Sdk1 and Sdk2 are single-pass transmembrane proteins, with extracellular regions composed of 6 N-terminal immunoglobulin (Ig) domains followed by 13 fibronectin type III (FNIII) domains, and a relatively short intracellular domain terminating in a Postsynaptic density/Discs Large/ZO-1 (PDZ) binding motif. Here, we report the crystal structures of cell-cell adhesive homophilic dimers of mouse Sdk1 and Sdk2, each mediated by the four N-terminal Ig domains. These four domains adopt a horseshoe conformation, like many other IgSF cell-cell recognition proteins, but they interact in a unique back-to-back anti-parallel manner not previously observed. Overall, our data suggest a model in which Sdks form cis dimers on isolated cell surfaces, which dissociate to form trans dimers through the same interface when contact is made to a cell surface expressing the cognate Sdk.

The Sdk1Ig1–5 structure showed that Ig5 extends laterally from the horseshoe with a 54° deviation from linearity with Ig4. This angle is maintained in both independent Ig1–5 chains observed in the crystal structure. The linker between Ig4 and Ig5 is only one amino acid (N379) and there is a small Ig4:Ig5 interface with a buried surface area (BSA) over both domains of ~370 Å2. This interface—involving the linker region, the Ig4 AB loop and the Ig5 BC loop—likely provides rigidity to the Ig4–Ig5 junction. Consistent with the AUC results of the wild-type Sdk1 and Sdk2, the crystal structures show a dimeric arrangement of molecules, consisting of symmetrical back-to-back interactions (convex-face to convex-face) between the Ig1–4 horseshoe regions of the individual protomers, with Ig5 making no contacts in the Sdk1Ig1–5 dimer. (A) Surface view of the Sdk1Ig1–5 structure showing the back-to-back horseshoe-mediated dimer observed in the crystal structure. The positioning of Ig6 is therefore unknown, however, since Ig5 projects away from the dimer interface it is unlikely Ig6 would be able to contribute to the dimer observed in the crystal structures, which is described in detail below. (G) Our data suggest Sdk dimerizes using the crystallographically-determined interface, both between molecules emanating from opposing cell surfaces (in trans)—mediating cell-cell interactions—and between molecules emanating from the same cell surface (in cis)—mediating Sdk clustering. These interactions are shown schematically, using the Sdk1Ig1–5 crystal structure to illustrate the dimer interaction.

>[2x]GPALAQDDVAPYFKTEPGLPQIHLEGNRLVLTCLAEGSWPLEFKWIRNDSELTTYSSEYKYIIPSLQKLDAGFYRCVVRNRMGALLQRKSEIQVAYMGNFMDTDQRKTVSQGHAALLNLLPIVSCPQPQVTWFREGHKIIPSSRIAITLENQLVILATTASDAGAYYVQAVNEKNGENKTSPFIHLSVARDTGTHEAMAPIIVVAPGNRSVVAGSSETTLECIANARPVEELSVHWKRNGVRLTSGLHSYGRRLTITNPTSADTGMYVCEATLRGSTFEPARARAFLSIIEPPYFTAEPESRILGEVEETMDIPCRAMGVPLPTLQWYKDAVPLSKLQNPRYKVLPSGGLHIQKLSPEDSGIFQCFASNEGGEVQTHTYLDVTNIAPAFTQRPVDTTVTDGMTAVLRCEVSGAPKPAITWKRGNHILASGSVRIPRFMLLESGGLRIAPVFIQDAGNYTCYAANTEASVNASAMLTVWNRT> MAAAAVVAATVPAQSMGADGASSVHWFRKGLRLHDNPALLAAVRGARCVRCVYILDPWFAASSSVGINRWRFLLQSLEDLDTSLRKLNSRLFVVRGQPADVFPRLFKEWGVTRLTFEYDSEPFGKERDAAIMKMAKEAGVEVVTENSHTLYDLDRIIELNGQKPPLTYKRFQALISRMELPKKPAVAVSSQQMESCRAEIQENHDDTYGVPSLEELGFPTEGLGPAVWQGGETEALARLDKHLERKAWVANYERPRMNANSLLASPTGLSPYLRFGCLSCRLFYYRLWDLYKKVKRNST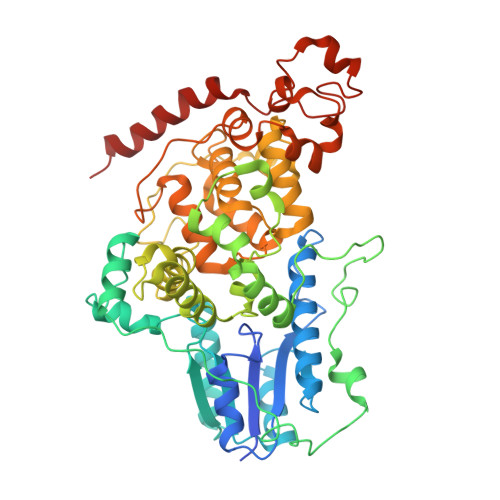PPLSLFGQLLWREFFYTAATNNPRFDRMEGNPICIQIPWDRNPEALAKWAEGKTGFPWIDAIMTQLRQEGWIHHLARHAVACFLTRGDLWVSWESGVRVFDELLLDADFSVNAGSWMWLSCSAFFQQFFHCYCPVGFGRRTDPSGDYIRRYLPKLKGFPSRYIYEPWNAPESVQKAAKCIIGVDYPRPIVNHAETSRLNIERMKQIYQQLS> STRPPRFQRDFVDLRTDCPSTHPPIRVMQWNILAQALGEGKDNFVQCPVEALKWEERKCLILEEILAYQPDILCLQEVDHYFDTFQPLLSRLGYQGTFFPKPWSPCLDVEHNNGPDGCALFFLQNRFKLVNSANIRLTAMTLKTNQVAIAQTLECKESGRQFCIAVTHLKARTGWERFRSAQGCDLLQNLQNITQGAKIPLIVCGDFNAEPTEEVYKHFASSSLNLNSAYKLLSADGQSEPPYTTWKIRTSGECRHTLDYIWYSKHALNVRSALDLLTEEQIGPNRLPSF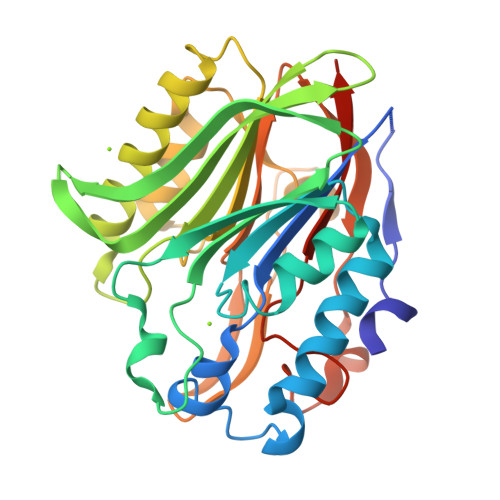NYPSDHLSLVCDFSFTEESDGLS A prominent member of the PspA family is the vesicle-inducing protein in plastids 1 (Vipp1), also known as IM30 (inner membrane-associated protein of 30 kDa). Vesicle-inducing protein in plastids 1 (Vipp1) is critical for thylakoid membrane biogenesis and maintenance. Vipp1 appears to have two functions: in membrane maintenance (that is, during heat or light stress) and in thylakoid membrane (TM) biogenesis and/or remodeling. Vipp1 binds to negatively charged membranes and membrane binding depends on stored curvature elastic stress.

By analyzing ten additional unique structures of N-terminally truncated Vipp1 in the presence of lipids, we show that helix α0 is a major determinant for the types of polymeric assemblies that are formed by Vipp1 and that helix α0 serves as a membrane anchor for Vipp1. To obtain more insights into its function, we analyzed the interaction of a truncated Vipp1 lacking α0 (Vipp1 (α1–α6)) with membranes using cryo-EM. We found that, in the absence of α0, Vipp1 forms PspA-like rods that are not capable of membrane tubulation and apparently do not interact with membranes. Thus, α0 is critical for membrane interaction and tubulation of Vipp1 and in controlling the polymer architecture of Vipp1. Membrane tubulation of Vipp1 is largely mediated by α0, as truncated Vipp1 (α1–α6) assembled into helical tubes that did not internalize any lipid membrane in the lumen. Although it has been reported that truncated versions of Vipp1 lacking α0 are still capable of membrane binding, our micrographs and cryo-EM maps show that Vipp1 (α1–α6) does not engulf membranes in the rod lumen and does not assemble on membranes, while it may still be capable of binding lipids in other conditions. Moreover, the truncation of helix α0 also affects the assembly state of Vipp1. Additionally, the monomer orientation and rod symmetry differ from the rods observed upon incubation of the full-length protein with membranes while the Vipp1 (α1–α6) rods adopt a SynPspA rod-like symmetry and orientation and cover a large range of diameters. In the PspA-like Vipp1 (α1–α6) rods, however, a register shift and a larger distance to the next layer of monomers would make it impossible for α0 to reach α1 + α4 of the monomer in the adjacent layer. Thus, the presence and absence of α0 coordinates different assembly states of Vipp1 and interactions of helix α0 stabilize particular polymeric Vipp1 structures.

> DPEKVLEQAVIDMQEDLVQLRQAVARTIAEEKRTEQRLNQDTQEAKKWEDRAKLALTNGEENLAREALARKKSLTDTAAAYQTQLAQQRTMSENLRRNLAALEAKISEAKTKKNMLQARAKAAKANAELQQTLGGLGTSSATSAFERMENKVLDMEATSQAAGELAGFGIENQFAQLEASSGVEDELAALKA>[2x]MENENKPNVANFEAAVAAKDYEKACSELLLILSQLDSNFGGIHEIEFEYPAQLQDLEQEKIVYFCTRMATAITTLFSDPVLEISDLGVQRFLVYQRWLALIFASSPFVNADHILQTYNREPNRKNSLEI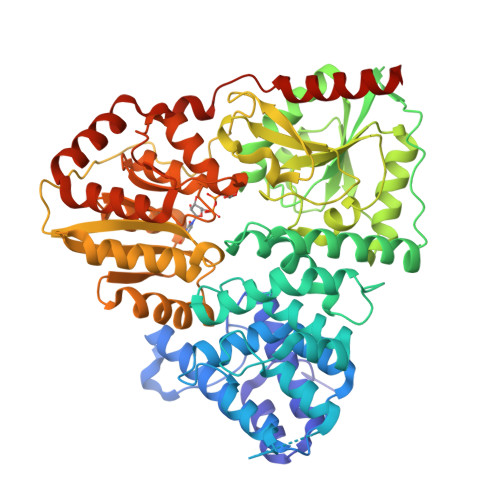HLDSSKSSLIKFCILYLPESNVNLNLDVMWNISPELCASLCFALQSPRFVGTSTAFNKRATILQWFPRHLDQLKNLNNIPSAISHDVYAHCSYDTSVNKHDVKRALNHVIRRHIESEYGWKDRDVAHIGYRNNKPVMVVLLEHFHSAHSIYRTHSTSMIAAREHFYLIGLGSPSVDQAGQEVFDEFHLVAGDNMKQKLEFIRSVCESNGAAIFYMPSIGMDMTTIFASNTRLAPIQAIALGHPATTHSDFIEYVIVEDDYVGSEECFSETLLRLPKDALPYVPSALAPEKVDYLLRENPEVVNIGIASTTMKLNPYFLEALKAIRDRAKVKVHFHFALGASNGITHPYVERFIKSYLGDSATAHPHSPYHQYLRILHNCDMMVNPFPFGNTNGIIDMVTLGLVGVCKTGAEVHEHIDEGLFKRLGLPEWLIANTVDEYVERAVRLAENHQERLELRRYIIENNGLNTLFTGDPRPMGQVFLEKLNAFLKENLEHHHHHH>SLMADEIAKAQVARPGGDTIFGKIIRKEIPAKIIFEDDRCLAFHDISPQAPTHFLVIPKKHISQI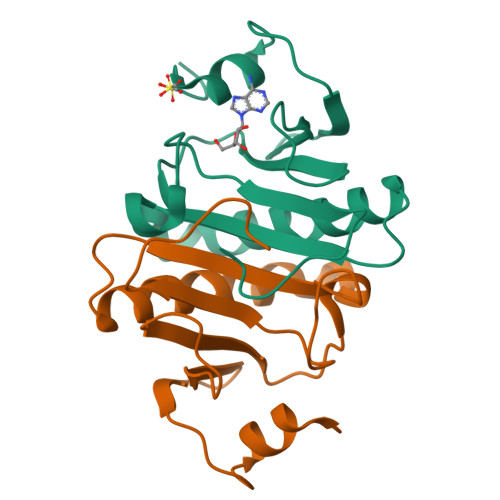SVAEDDDESLLGHLMIVGKKCAADLGLNKGYRMVVNEGSDGGQSVYHVHLAVLGGRQMHWPPG[4x]>MLQVDIGSTSGKAGSVVSVPITFTNVPKSGIYALSFRTNFDPQKVTVASIDAGSLIENASDFTTYYNNENGFASMTFEAPVDRARIIDSDGVFATINFKVSDSAKVGELYNITTNSAYTSFYYSGTDEIKNVVYNDGKIEVIALEHHHHHH[2x];>[2x]KFIYGDVDGNGSVRSIDAVLIRDYVLGKINEFPYEYGMLAADVDGNGSIKIND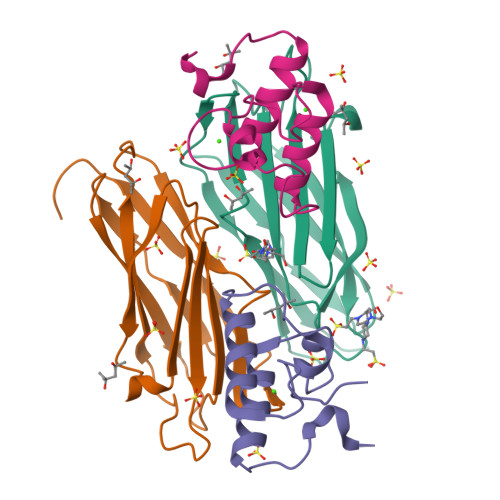AVLVRDYVLGKIFLFPVEEKEE>[2x]SNAKNTMPLVIAYNNAPEDDKIQKLFYLQKINYLLNKTQLNDDLFDWINDAEEGGWLNELAKFSINPNASFFLKGMQFAKAITEEIKNKPEINSSEVNIYHLMQERDQLLKEVEFEKCATRYAEINFLLNELALNDKKTKEIVERQTEILRLVAPKIKAIKGESIDNLPVIPSYKTKELGNHVNNFNFKFTMSGWEAPFVFRVEDRHELGKEQELHSYGVSKYFIEDYSVFMMRFKAEDGSTVYKPVILSQFANQNNLEEIAKQLKDGSPKNIAPRIGYYFVQLTDFCLKLIETHNYHPDIKLNNFLVHNNRVLVSDRKTFTTNDNPLASEILTSPLFAPDEFLKCLLFNKEGDPVGYNRNALWKRMNMPQFMAYQLGMALKQFLILTQLDELPD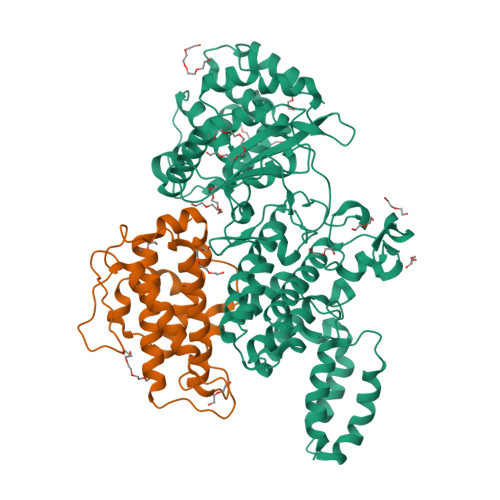DFRNPDHSAVSHFKTPSRQIINLSLLVQELTRLDPDKRMTIKQFQTLLNFKNLPPDAFYQKVEEVFPSSQLGIAEDIEALNKVLNSDLKGEALLKQANPVFTKLSKYDPKETRLTRLAEKLAIRCFNN;>SNAEATLGSGNLRQAVMLPEGEDLNEWIAVNTVDFFNQINMLYGTITEFCTEASCPVMSAGPRYEYHWADGTNIKKPIKCSAPKYIDYLMTWVQDQLDDETLFPSKIGVPFPKNFMSVAKTILKRLFRVYAHIYHQHFDSVMQLQEEAHLNTSFKHFIFFVQEFNLIDRRELAPLQELIEKLGSKDR[2x]>[4x]MDIKINDITLGNNSPFVLFGGICVLESLDSTLQTCAHYVEVTRKLGIPYIFKASFDKANRSSIHSYRGVGLEEGLKIFEKVKAEFGIPVITDVHEPHQCQPVAEVCDVIQLPAFLARQTDLVVAMAKTGNVVNIKKPQFLSPSQMKNIVEKFHEAGNGKLILCERGSSFGYDNLVVDMLGFGVMKQTCGNLPVIFDVTHSLQTRDAGSAASGG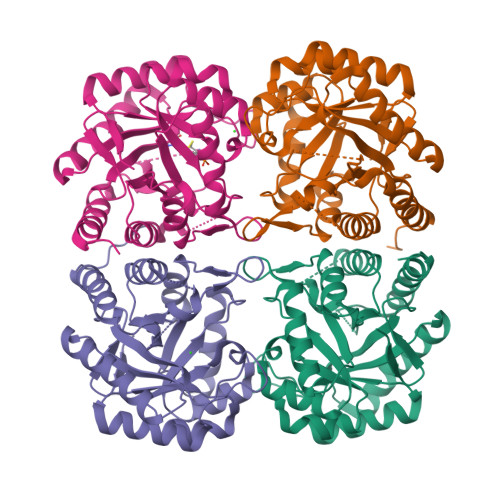RRAQALDLALAGMATRLAGLFLESHPDPKLAKCEGASALPLHLLEDFLIRIKALDDLIKSQPILTIE>[2x]MRSSHHHHHHSSGLVPRGSHMESKKDDTDLKLVSHNVYMLSTVLYPNWGQYKRADLIGQSSYIKNNDVVIFNEAFDNGASDKLLSNVKKEYPYQTPVLGRSQSGWDKTEG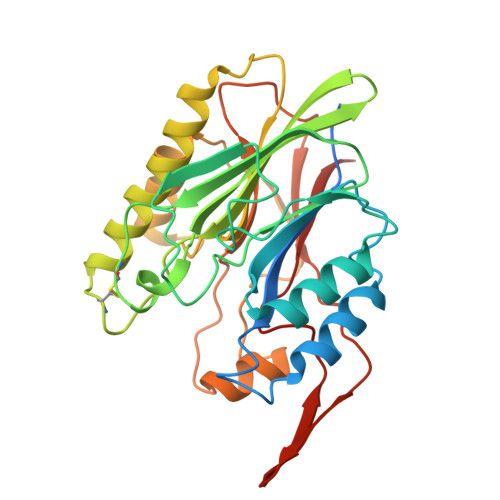SYSSTVAEDGGVAIVSKYPIKEKIQHVFKSGCGFDNDSNKGFVYTKIEKNGKNVHVIGTHTQSEDSRCGAGHDRKIRAEQMKEISDFVKKKNIPKDETVYIGGDLNVNKGTPEFKDMLKNLNVNDVLYAGHNSTWDPQSNSIAKYNYPNGKPEHLDYIFTDKDHKQPKQLVNEVVTEKPKPWDVYAAAYYYVYNDFSDHYPIKAYSK PHENOL | C6 H6 O | 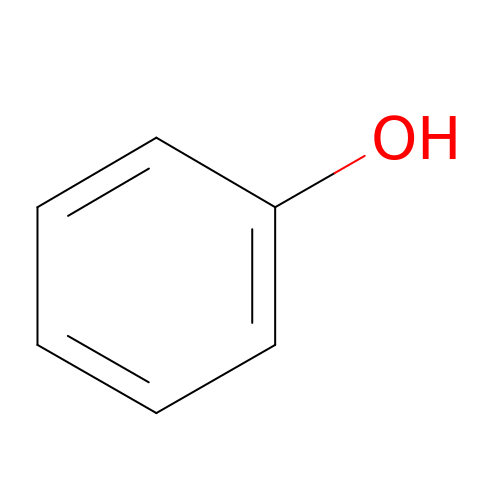ISWSIDIOOBJBQZ-UHFFFAOYSA-N>SNAMTEAMKITLSTQPADARWGEKATYSINNDGITLHLNGADDLGLIQRAARKIDGLGIKHVQLSGEGWDADRCWAFWQGYKAPKGTRKVVWPDLDDAQRQELDNRLMIIDWVRDTINAPAEELGPSQLAQRAVDLISNVAGDRVTYRITKGEDLREQGYMGLHTVGRGSERSPVLLALDYNPTGDKEAPVYACLVGKGITFDSGGYSIKQTAFMDSMKSDMGGAATVTGALAFAITRGLNKRVKLFLCCADNLISGNAFKLGDIITYRNGKKVEVMNTDAEGRLVLADGLIDASAQKPEMII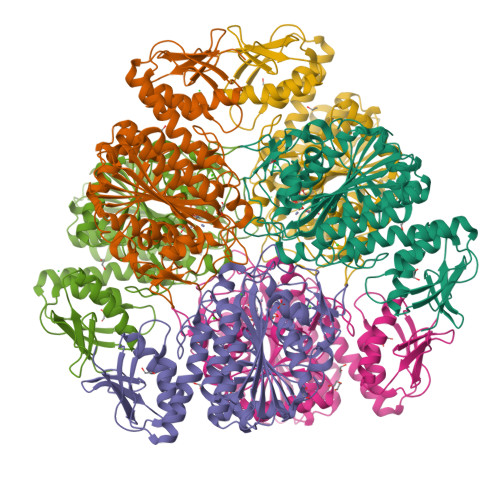DAATLTGAAKTALGNDYHALFSFDDALAGRLLASAAQENEPFWRLPLAEFHRSQLPSNFAELNNTGSAAYPAGASTAAGFLSHFVENYQQGWLHIDCSATYRKAPVEQWSAGATGLGVRTIANLLTA[12x]Prokaryotic sodium channels are homotetramers, in which each monomer contains six transmembrane segments and is homologous to a single eukaryotic pseudorepeat. As with the eukaryotic channels, their S1–S4 segments form the voltage sensors, and the S5–S6 segments from each polypeptide chain associate to form an eight‐helix bundle that constitutes the pore. The selectivity filter (SF), which determines the channel's Na+ permeability over other cations, is formed by the close association of the P loops from each of the polypeptide chains.

In this study, we analysed new crystals of the NavMs pore that contain only sodium ions and diffract to higher resolution (2.7 Å), enabling us to identify the sodium binding sites in the SF. The NavMs sodium channel pore protein was purified and crystals grown in the presence of sodium ions. The pores in these crystals are in the open conformation, with the activation gate at the intracellular ends of the transmembrane domains of all four monomers splayed to allow ions to exit the pore, as in Bagnéris et al (2013). The locations of three highly occupied sodium ion sites are seen in the centres of the selectivity filters, with ion B‐factors similar to those of the protein atoms. Densities attributable to partially occupied water molecules are distinct and can also be seen within the SF and at the bottom of the SF/top of the hydrophobic internal cavity close to the local anaesthetic channel blocker binding sites (Bagnéris et al, 2014). The sodium site nearest to the extracellular surface (NaI; top cyan ball in Fig 2A) is located close to the site that had been designated S1 in molecular dynamics studies of the NavMs pore (Ulmschneider et al, 2013). Below that is the site we designate as NaII, which is closest to the carbonyl oxygen of Leu177, and is separated from the NaI site by ~2.8 Å. NaIII corresponds closely to the site denoted S4 in the MD studies and above the proposed SiteIN. It is nearest to the carbonyl oxygen of Thr176; it is separated from NaII by ~5.6 Å. An important finding is that there are no protein atoms within the normal outer limit (3.5 Å) for a sodium ion coordination sphere (the closest is Oγ1 of Ser179 at 3.79 Å from NaI), suggesting that protein–ion interactions are mediated by intermediate water molecules.

>GSHMGVGSVAALLTVVFYIAAVMATNLYGATFPEWFGDLSKSLYTLFQVMTLESWSMGIVRPVMNVHPNAWVFFIPFIMLTTFTVLNLFIGIIVDAMAITKEQEEEAKTGHHQEPISQTLLHLGDRLDRIEKQLAQNNELLQRQQPQKK[4x]>MASKPIEDYGKGKGRIEPMYIPDNTFYNADDFLVPPHCKPYIDKILLPGGLVKDRVEKLAYDIHRTYFGEELHIICILKGSRGFFNLLIDYLATIQKYSGRESSVPPFFEHYVRLKSYQNDNSTGQLT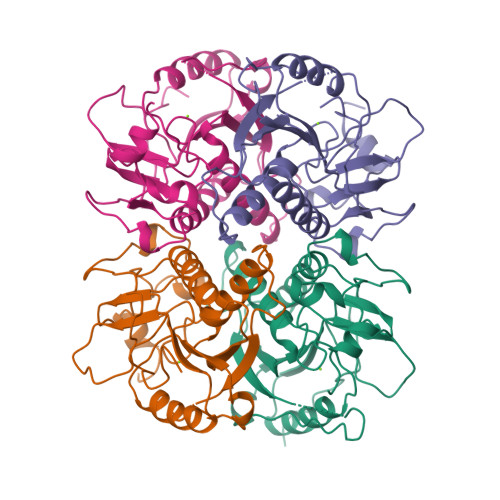VLSDDLSIFRDKHVLIVEDIVDTGFTLTEFGERLKAVGPKSMRIATLVEKRTDRSNSLKGDFVGFSIEDVWIVGCCYDFNEMFRDFDHVAVLSDAARKKFEKV[4x]>[2x]MFKTEFEFPEELKTKLQEHINYFPKKRQAILLCLHEIQNYYGYIPPESLKPLADMLELPLNHVEGVVAFYDMFDREDKAKYRIRVCVSIVCHLMGTNKLLKALENILGIKPGEVTPDGKFKIVPVQCLGACSEAPVFMVNDDEYKFESEVQLNEILSRYT;>MRSYPAIPRIYAETTLNMLLKRAKKPRVHSIDEYLKDGGYQALEKALNMSPEEIIDWVDKSTLRGRGGAGFPTGKKWKFAVQNPGPRYFICNADESEPGTFKDRIIIERDPHLLIEGIIISSYAIGANEAYIYIRGEYPAGYYILRDAIEEAKKKGFLGKNILGSGFDLEIYVARGAGAYICGEETALIESLEGKRGHPRLKPPYPVQKGLWGKPTVVNNVETIANVPFIISMGWEEYRYIGPSDYAGPKLFPVSGKVKKPGVYELPMNT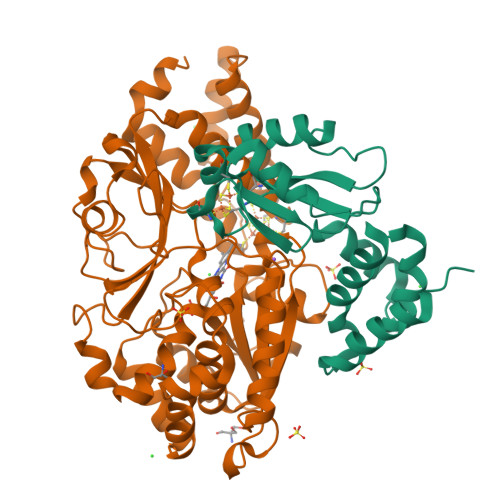TLREVIFKYAGGTLGNKKVKAVFSGALDCFSSEELDIPMDYSPLGFGGTGTVIVLTEEDDIVEAALKIAEFYEHETCGQCTPCRVGCYEQANLLEKIYKGEATEQDWEGFDFVNRNIQPTSICGLGAVAGRLIRQTLEKFPEEWEKYRKKSASLPLAGHHHHHH[2x]> GPLGSMNDRADFVVPDITTRKNVGLSHDANDFTLPQPLDRYSAEDHATWATLYQRQCKLLPGRACDEFLEGLERLEVDADRVPDFNKLNEKLMAATGWKIVAVPGLIPDDVFFEHLANRRFPVTWWLREPHQLDYLQEPDVFHDLFGHVPLLINPVFADYLEAYGKGGVKAKALGALPMLARLYWYTVEFGLINTPAGMRIYGAGILSSKSESIYCLDSASPNRVGFDLMRIMNTRYRIDTFQKTYFVIDS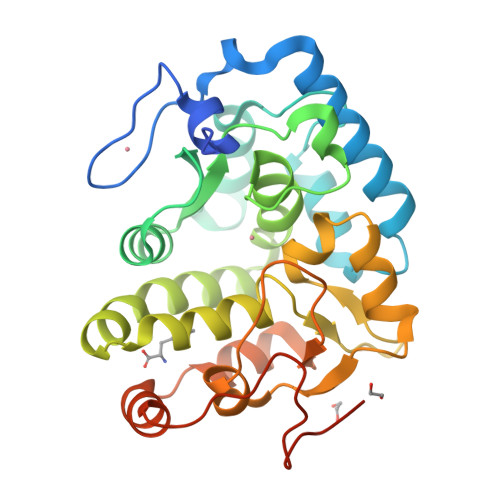FKQLFDATAPDFAPLYLQLADAQPWGAGDIAPDDLVLNAGDHQGWADTEDV RanBP3 is a Ran-interacting protein with diverse roles in nuclear transport. Specifically, RanBP3 enhances the rate of NES export by increasing the affinity of CRM1 for RanGTP, thereby stabilizing the ternary CRM1/Ran/cargo complex in the nucleus. RanBP3 belongs to a class of Ran-binding proteins characterized by one or more Ran-binding domains (RBDs) of approximately 120 residues. As expected, the RanBP3 RBD adopts a pleckstrin homology fold, composed of 7 anti-parallel β-strands and a C-terminal α-helix.

We therefore pursued the structure of the RBD in its unbound form. We solved the structure at 1.61 Å resolution using experimental phases obtained from a platinum derivative, and at 2.1 Å in a second crystal form by molecular replacement. Crystal forms 1 and 2 contain two and four molecules per asymmetric unit, respectively, and aligning these structures reveals variations in the N- and C-terminal residues and in several loops, reflecting the inherent flexibility of these regions. In contrast, the β5β6 loop, whose functional role is evoked below, is highly uniform in structure, suggesting a comparatively rigid element. The strands define a continuous sheet with simple up-down topology, forming an imperfect β barrel that juxtaposes strands 4 and 6 and extrudes strand 5. The C-terminal helix caps the barrel, packing against strands 1, 2, 5 and 6.

>GAMKVEVITGEEAESNVLQMQCKLFVFDKTSQSWVERGRGLLRLNDMASTDDGTLQSRLVMRTQGSLRLILNTKLWAQMQIDKASEKSIRITAMDTEDQGVKVFLISASSKDTGQLYAALHHRILALRSRVEQEQEAK[4x]>SNAMEDLDALWERYREAVRAGGNPQALYQEMVWPALLALWREKPRVYPFPQAFAVSVHTLGTSPEATALAILGAGAERVYVLHTPESARFLPRLRQDTGKDLYPVEIGKSDVEAIYREVKRLLEKHPEVPVALDLTSGTKAMSAGLAAAGFFFQRFYPKVRVVYVDNEDYDPELRRPRAGTEKLRILPNPHEALAEVDALFAKELYGKGEFGQAAAYFRGMVGRTGNQAYALYALLAEMYRAWRALDFGEALKAGRKLLGQLSQNVWLNHPLNARRE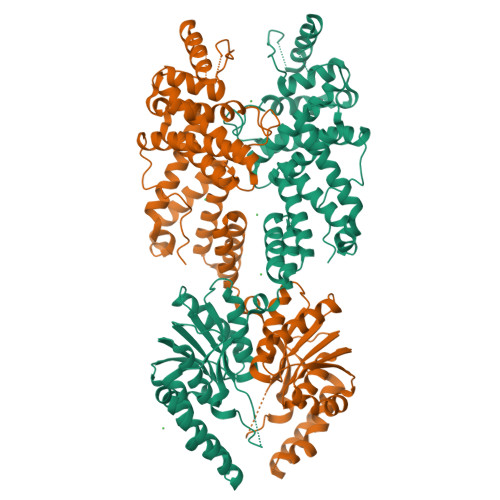ALEAQVALLEAVDRFLKARDFALKEGVYGLARTLLHLAQEAKEEAAVLAALYAYRALELLLQERLALLGRRAEAPGLSPEEAEALRKALAELLGVLPEEVRLPAKLGLLDLLAFLRLKGDEALGRLSLAELRGLAGALKGRNSALLVHGFDVPSPKAVEGIARLAQGLLQDLEARTALGPLSPEPVPLGF[2x]> MSYSAYFAKAGFQFPAGLSALVAGIVALNVCTGRPTKGTKEISNAEYNATPIGYLQSPDQHPTAFPKVPGMKDVHGSPHHHH;> MMRAAQKAKQELPATVLTQTRSYLAPLRSDFTEEITAPKVASASNLVNEWNNKKQATENLMKLLQAYKDIGDAKSEPLLKNHNPRTFEDRDYPVPDFRTQNLKAGDVPKFFDTVISTRASAAIASKDKFWAGRKTEAEAASAKASAAFPRVAVPEWKKGKTVSIENLNTVTDKYAAALVPKRKLALPVLPEGVKKAVEDFAASVGQAKNASEVSELLAKSLAEKAVVTEGGKVVEGFSYVSKAVAAKVIATRRAEVHERLLKLWAKRLLVSPELAIVPLNEFDAQLASKFEGISPKYQELLSAVAQGNKTFAQRLNSSPAFSSFLLKREKAESEVPPSELELEAAQKAAELEDPEVALRTLLGPQMEALGASDLLLSEQIRVITEHRYTPDRLQYKEGMKLADKIAAQEAALKEELKVIYGDNVDVKHFQASPRTPVQQLFDSLKNAAANKERAAKEAAAAASPYLAYAVTKKQEVQADPSNIPFDEVLYPQLSEELLELELSDIREDEIALEKAEEEELWLLTLTQQFKHIQKHFGIDLPHSVVAHMDPLLIKKIDWETTNALEDFDITLDDMGAEDAKEQWGAENLSHHFLPLIRYRRDLARKNGDRYGPDLVNGN;> MRQASRLALSIRQAGNVEAASAVPAMTRQFSAPGSHEHHETPLSKVMPTVVSIPRKVACLALGATKKVVCGLASSGPSQNLVSTFANKVIVEENLVNVAEIDVPFWSYWLSSAGFTSKDAFVKFAEAVKPKVAALSTSDITNLTVAFKRANYYDKDLFTGIEANVSANFTKFETEQLLQIVATFDAFNHSSVAFLDDVADSITYCNHYLAPVRAGADELATLLTYYAKNGHERADLLATVARGFSEVSLGKLSAAQRKDTVLSALKAFQTFGFYPESIEAVIGAALVSPAEYSAEELKEVEAVKVAAENALGGEFVLIQEGAHGH;> MKLLPESLQQEAATAAVVASWVLWHLDTQLLPTIMREHKLHACWAAAAKRYNEKLFKLNPSYDRVLSLPAVSKNQVLENVFHTAPKAPVEHLEKMVSANSKVYDALNLQSKRVLIWQVKPALF;> MMLRTLTRSSAVAGQA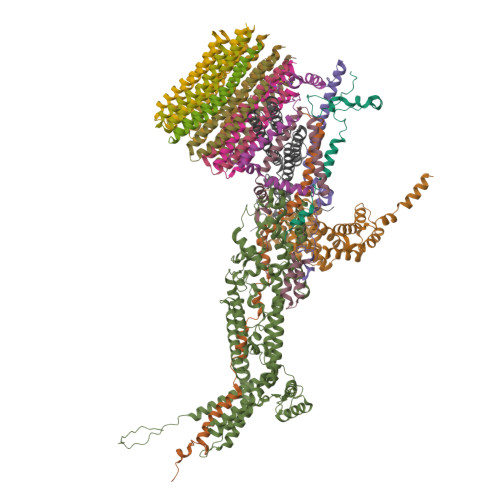VRLFKTSAAAAEGNSVAGIIKSVNETSGANLLSSLKTIKAQAAPIYPAAASSTGYSTQAKIALFGALSWILYRADGQSKAHEWIVDLNLNVLQAAWLISFSSLIPFRAVYFAFRGMAPATASTLNGLKTFSSISL;> MVLGEVYLKDILRTPPTGAIPANVPHPFQTSFYTYATKKLIPRHWYLLGGFTFTITLYGILDGLRDSGKKKAYDEAIHAGKTPYTAGGH;> MAVTSFLGKAFEKYFYDFSAYEQFGLNRFLSSKGQYVALRHVGFVMVGVNVLLAANFPFNPPFPTIGMCPAGWEGTWVCQADKAKALEMYKEWKKSN;>MSVQRLSLGAARCLSAGVARVQASQALVAQKAVAVAPTRAQAAPAEVAQVRSMSVLAASKMVGAGCATIALAGVGAGLGVMFGSLINGAARNPNIAKQLVGYALLGFALTESIALFSLLVVFLILFA[10x];> MSVLSSVSMGSRIGSSLLGRSSAYLAQCGFSTRSNLNGSIDTSSSVFQALSSDNENKPAASPLNVKLPGMSCSSILLPKTSRIAVPFGNQTMAMSSVRDVKTGSLPTNFLTGVYRFWRSQNPAEKPHDPVNDRLLPAVVDASDKRASIGTWATTFFCTIISCNLLGLMPFNEAPTSGLGFATGLGVSVWATATILGLSKTGFKFPGHFIPGGTPWPMAFIFVPLETISYTFRAVSLGVRLWVNMLAGHTLLHILTGMALALPFSLGFFSMVPATFGVCCLLSALVGLEYLVAVLQSGVFSILSTVYVGEFNHDKFIGPAAKIVKKIH>[5x]TASLVEGVELTKYISDINNNTDGMYVVSSTGGVWRI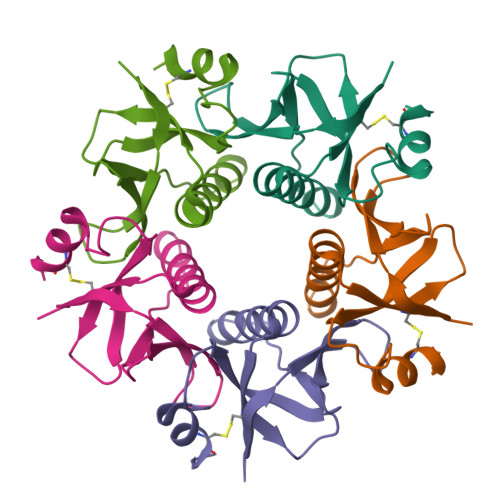SRAKDYPDNVMTAEMRKIAMAAVLSGMRVNMCASPASSPNVIWAIELEAEGSGSGASQFFKDNCNRT> MKYMITSKGDEKSDLLRLNMIAGFGEYDMEYDDVEPEIVISIGGDGTFLSAFHQYEERLDEIAFIGIHTGHLGFYADWRPAEADKLVKLLAKGEYQKVSYPLLKTTVKYGIGKKEATYLALNESTVKSSGGPFVVDVVINDIHFERFRGDGLCMSTPSGTTAYNKSLGGALMHPSIEAMQLTEMASINNRVYR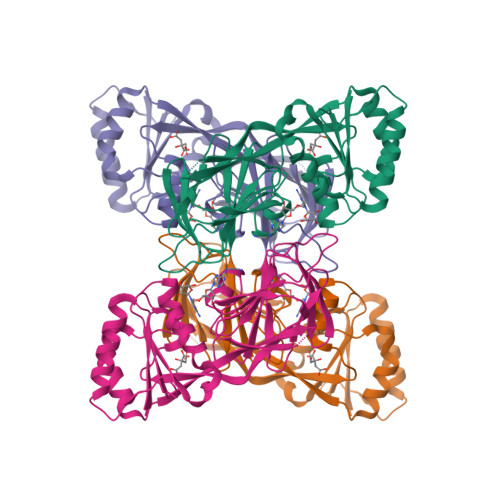TIGSPLVFPKHHVVSLQPVNDKDFQISVDHLSILHRDVQEIRYEVSAKKIHFARFRSFPFWRRVHDSFIEDLEHHHHHH> GGAGAGGAG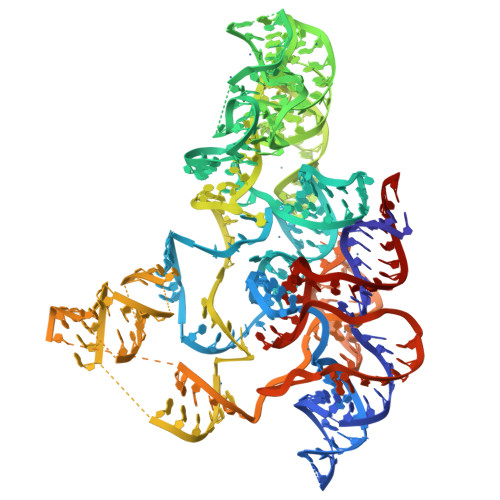CAGGCGGUCGCGGGGGCGCACACCUGCGCUUCCCGAGGAAAGUCCGGACUCUGGAGCGGGGUGCCGGGUAACGCCCGGGAGGGGUGACCCUCGGACAGGGCCAUAGAGAAGAAGACCGCCCGUUGAGGGCAAGGGUGGAACGGUGGGGUAAGAGCCCACCAGCGUCGGGGCAACCCGGCGGCUUGGCAACCCCCACCUGGAGCAAGGCCAAGCAGGGGGUUGGGUCGCUCCCCCUAUUCCCCCGGGUUGGCCGCUUGAGGUGUGCGGUAACGCACACCCCAGAUUGAUGACCGCCCACGACAGAAUCCGGCUUAUGCUCCUCUCCCGUG>MAKSKFEYVRDFEADDTCLAHCWVVVRLDGRNFHRFAEKHNFAKPNDSRALQLMTKCAQTVMEELEDIVIAYGQSDEYSFVFKRKTNWFKRRASKFMTHVASQFASSYVFYWRDYFEDQPLLYPPGFDGRVVVYPSNQTLKDYLSWRQADCHINN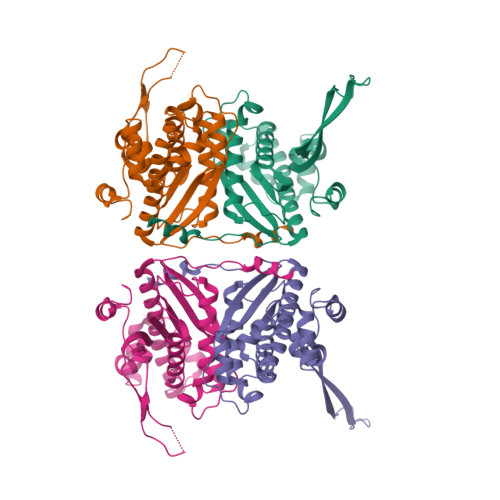LYNTVFWALIQQSGLTPVQAQGRLQGTLAADKNEILFSEFNINYNNELPMYRKGTVLIWQKVDEVMTKEIKLPTEMEGKKMAVTRTRTKPVPLHCDIIGDAFWKEHPEILDEDS[2x]>[2x]VIEKVQHIQLLQKNVRAQLVDMKRLEVDIDIKIRSCRGSCSRALAREVDLKDYEDQQKQLEQVIAK;>[2x]HQLYIDETVNSNIPTNLRVLRSILENLRSKIQKLESDVSAQMEYCRTPCTVSCNIPVVSGKECEEIIRKGGETSEMYLIQPDSSVKPYRVYCDMNTENGGWTVIQNRQDGSVDFGRKWDPYKQGFGNVATNTDGKNYCGLPGEYWLGNDKISQLTRMGPTELLIEMEDWKGDKVKAHYGGFTVQNEANKYQISVNKYRGTAGNALMDGASQLMGENRTMTIHNGMFFSTYDRDNDGWLTSDPRKQCSKEAGGGWWYNRCHAANPNGRYYWGGQYTWDMAKHGTDDGVVWMNWKGSWYSMRKMSMKIRPFFPQQ;>YEASILTHDSSIRYLQEIYNSNNQKIVNLK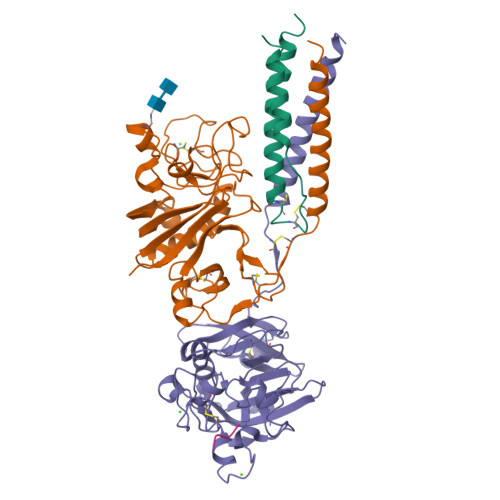EKVAQLEAQCQEPCKDTVQIHDITGKDCQDIANKGAKQSGLYFIKPLKANQQFLVYCEIDGSGNGWTVFQKRLDGSVDFKKNWIQYKEGFGHLSPTGTTEFWLGNEKIHLISTQSAIPYALRVELEDWNGRTSTADYAMFKVGPEADKYRLTYAYFAGGDAGDAFDGFDFGDDPSDKFFTSHNGMQFSTWDNDNDKFEGNCAEQDGSGWWMNKCHAGHLNGVYYQGGTYSKASTPNGYDNGIIWATWKTRWYSMKKTTMKIIPFNRLTIGEGQQHHLGGAK[2x];>[2x]GHRP>MAKESVKILQGKLDVKSLIDQLNAALSEEWLAYYQYWVGALVVEGAMRADVQGEFEEHAEEERHHAQLIADRIIELEG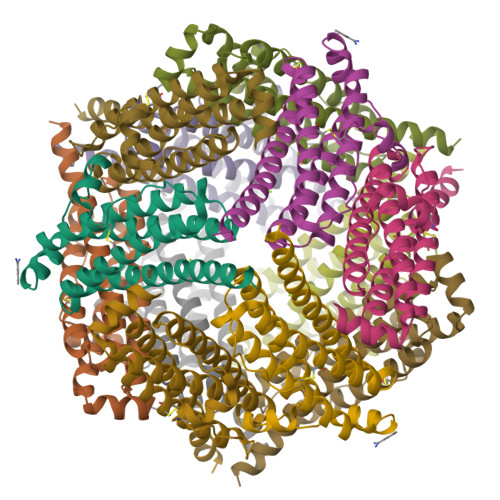VPVLDPKKWFELARCKYDSPTAFDSVSLLNQNVSSERCAILRYQEIANFTNGKDYTTCDIAKHILAEEEEHEQDLQDYLTDIARMKESFLKK[4x]> GSVYLRYFKGLILSDAYAPGLKWSDELKAYSALAFKYRDVRKYFLEKEIEVEENVIDSLPFPLIKDKIELRDYQAEAVKAWLKEKRGIIVLPTGAGKTQVALKIVSIMKVATLIVVPTIDLITQWKERINKYLDFDPGIIGGGEDSLKGITVITYDSAYTRAEELGNKFPLLIFDEVHHLPSEGYSIMAQLFASPYRLGLTATPERDDGKHELYPILV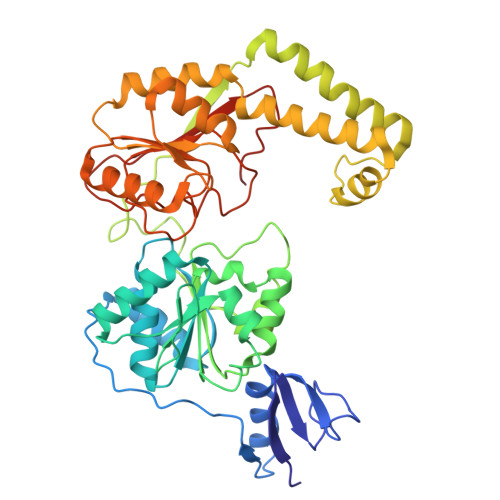GPIVYRKSVEELAGKYIAKYKIKKLYVSLTNEEKKRYDGLRKKLKDFLSSRGLKLQNLDDFHRLVKLAAKDKEAREALLAWHESLNIAVNSQSKIEKLREILQEYKNEKIIVFTRDTQMAYRISKTFLIPVVTYKTDKDEREEILQKFRDGEYRVIVASTVFDEGVDVPDATLAIVMGGYGTKRQFLQRLGRILRKKDKEALLIEIVTKGTADYRLSRRRRE> ASVKDTYTDRLDDWNGIIAGNQYYDSKNDQMAKLNQELEGKVADSLSSISSQADRIYLWEKFSNYKTSANLTATYRKLEEMAKQVTNPSSRYYQDETVVRTVRDSMEWMHKHVYNSEKSIVGNWWDYEIGTPRAINN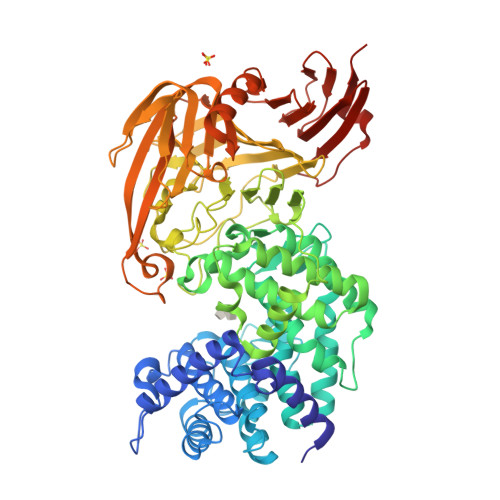TLSLMKEYFSDEEIKKYTDVIEKFVPDPEHFRKTTDNPFKALGGNLVDMGRVKVIAGLLRKDDQEISSTIRSIEQVFKLVDQGEGFYQDGSYIDHTNVAYTGAFGNVLIDGLSQLLPVIQKTKNPIDKDKMQTMYHWIDKSFAPLLVNGELMDMSRGRSISRANSEGHVAAVEVLRGIHRIADMSEGETKQRLQSLVKTIVQSDSYYDVFKNLKTYKDISLMQSLLSDAGVASVPRTSYLSAFNKMDKTAMYNAEKGFGFGLSLFSSRTLNYEHMNKENKRGWYTSDGMFYLYNGDLSHYSDGYWPTVNPYKMPGTTETDAKRADSDTGKVLPSAFVGTSKLDDANATATMDFTNWNQTLTAHKSWFMLKDKIAFLGSNIQNTSTDTAATTIDQRKLESSNPYKVYVNDKEASLTEQEKDYPETQSVFLESSDSKKNIGYFFFKKSSISMSKALQKGAWKDINEGQSDKEVENEFLTISQAHKQNRDSYGYMLIPNVDRATFNQMIKELESSLIENNETLQSVYDAKQGVWGIVKYDDSVSTISNQFQVLKRGVYTIRKEGDEYKIAYYNPETQESAPDQEVFKKLEQHHHHHH Rspo (R-spondin, also roof plate-specific spondin) proteins are evolutionarily conserved from fish to humans and have well-documented roles in a broad range of developmental and physiological processes resulting from enhancement of canonical and non-canonical Wnt signalling. ZNRF3/RNF43 specifically targets these Wnt receptors for ubiquitination and turnover, hence reducing Wnt signalling responses. Direct extracellular interaction with Rspo proteins inhibits ZNRF3/RNF43 activity. Here we report a molecular level analysis of the ZNRF3/RNF43 ectodomain structure and its interactions with Rspo proteins.

The crystal structures of the ZNRF3ecto–Rspo2Fu1–Fu2 and RNF43ecto–Rspo2Fu1–Fu2 complexes revealed a 1:1 interaction between Fu1 of the Rspo2Fu1–Fu2 and a single ZNRF3ecto or RNF43ecto chain. Neither the Rspo2Fu1–Fu2 nor the ZNRF3ecto dimer show major conformational changes on complex formation. The first, extensive, area of interaction involves hydrophobic interactions interspersed with hydrophilic (complementarily charged) patches contributed by the first two β-hairpins of the Rspo Fu1 and the region immediately carboxy-terminal to the β3 strand of ZNRF3ecto. The Met-finger at the tip of the second β-hairpin of Fu1 nestles into a pocket formed between the β3 strand and the αC–β7 loop of the ZNRF3ecto, which is lined with hydrophobic residues (I95, I191, V192, A198). The αC–β7 loop is a flexible region in the unliganded ZNRF3ecto crystal structures and moulds to interface the RspoFu1–Fu2 M68 in the complex. The acidic region of the β3–β4 loop (immediately adjacent to C104 of the disulphide bridge) becomes more ordered in the ligand-bound ZNRF3ecto structures, probably as a result of electrostatic interactions with a positively charged patch on Rspo Fu1. For all ZNRF3ecto–Rspo2Fu1–Fu2 complex structures we determined (from five different combinations of species and crystal forms), the dimer found in most of the unliganded ZNRF3ecto crystal structures reoccurs. The overall assembly thus comprises a 2:2 complex of ZNRF3ecto–Rspo2Fu1–Fu2. The 2:2 complex resembles a crab with the ZNRF3ecto dimer forming the body from which the two Rspo2Fu1–Fu2 ligands diverge, without interacting with each other, as the pincers. Notably, the β1–β2 hairpin shows less conformational variation in the liganded ZNRF3ecto dimer structures, always maintaining a tight embrace, consistent with the Rspo2Fu1–Fu2 interactions contributing an indirect stabilizing effect on the dimer via the β3–β4 loop.

>[4x]ETGKETAFVEVVLFESSPSGDYTTHTTGLTGRFSRAGAMLSAEGEIVQMHPLGLCNNNDEEDLYEYGWVGVVKLEQPELDPKPCLTVLGKAKRAVQRGATAVIFDVSENPEAIDQLNQGSEDPLKRPVVYVKGADAIKLMNIVNKQKVARARIQHLGTKHHHHHH;>ETGGTNPICKGCLSCSKDNGCLRCQPKLFFYLRREGMRQYGECLQSCPPGYYGVRGPDMNRCSRCRIENCDSCFSRDFCIKCKSGFYSHKGQCFEECPEGFAPLDDTMVCVDGTKHHHHHH[4x]> MLRRAPCLLATNIPRSAWDPAHFNTNWSDSYSTEIAARRHWPAKKWSIGLEPRTPRDWLQFSYRNLAYAYNGALRACQSFPEMLVCYKEMKQRGVKVDVDTMNVLLTRAARYERIQVDDVFLLFDELTALGARPDIAAVETLHTVLDHSAAMPYEWREARRRQLVELYNCLAMEEIERLAPHRVDRLLKEQIKRYRDNLRALKASLSPSVYRRYLHTMHSASMLLEEVHNFLWELVESDHPAMEIPALQLRIPFVGSVMRRPETDTNEKLVKYTDFEDTDVCSVFLAAAERAVDADLHDTRAVSERRIFLSLLTMISYSGVLYTSDLMAQLMEMVKYSTHASSRDSDAQRLLRYAVRGSSAAQDDLYRSLWLKVEMVADSRVLGRYIGAREPWSPIRVCFDERGLFKSYPPLVHASAKKTSAIEADATSGSGSTTMEEEQRQQSERQRMSTEITSHTSKGGEEMVEGVRGAVVAETSEASGVKDVALQEASHGEQRTVEALDLRWGDIHRLIERT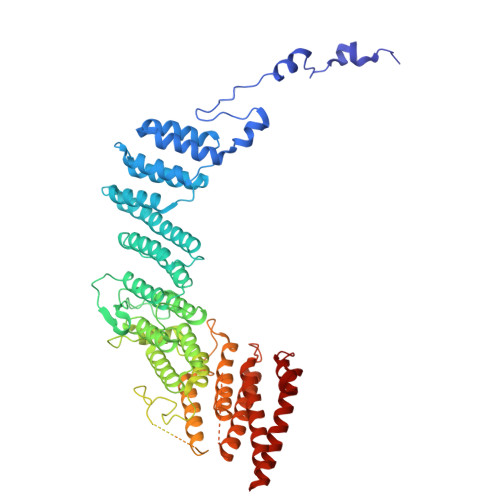RALTSPPTERHPQQEKMEIFTGIAVYLRTIATGRRYCSGEEEAGGESPAESRERALFAVGYELDVWARLFELVQEVRHDMEKFITDNAAHHVEPEFECWEALLITLRCILDFCVVRTQEKGKEERAAVEELFEKTMKLRNELVEESRTRFGGRMRILWLQEA Unspecific peroxygenases (UPOs) are a class of heme‐thiolate oxygenases from fungi that have similar catalytic scope to P450s, but are dependent only upon hydrogen peroxide (H2O2) as the external oxidant. A recent survey by Faiza and co‐workers explored the diversity of UPOs within sequence databases and was able to identify two major groups of enzymes: ‘long’ UPOs (Group I), typified by AaeUPO, of approximately 45 kDa molecular weight, and ‘short’ UPOs (Group II), typified by the enzyme from Marasmius rotula (MroUPO), which are of approximately 29 kDa. In this study, we have cloned the gene encoding an ‘artificial’ short UPO (artUPO) close in sequence to MroUPO, and expressed it in both Pichia pastoris and E. coli. In addition to their overall similarities in fold, artUPO, MroUPO and HspUPO feature both a glutamic acid and histidine residue (E164 and H93 in artUPO) that forms the catalytic acid‐base pair, in common with CPO and in contrast to the Glu‐Arg dyad found in AaeUPO.

We first crystallized artUPOyeast and determined the structure of the enzyme in two forms: the first in space group P212121, to a resolution of 2.01 Å and the second in C2221, to 1.21 Å, with two and one molecules in the asymmetric unit, respectively. The higher resolution structure in the C2221 space group superimposed with the monomer of the P212121 structure with an rmsd of 0.23 Å over 231 C‐alpha atoms, again indicative of high structural similarity, although clearly the higher resolution presents the enzyme structure in more detail with respect to water structure and alternate conformations of amino acids, which include D61 in the 1.21 Å structure. The structures confirm that each is a member of the short class of UPOs as defined by Faiza and co‐workers. The side chain amine of K156 H‐bonds with the backbone carbonyl groups of G89 and T90 in artUPOyeast, and may also confer extra stability to the enzyme. The differences between the active site tunnels of artUPOyeast and AaeUPO‐PaDa‐I are also noteworthy. artUPOyeast is distinguished from AaeUPO by the replacement of characteristic phenylalanine residues in that enzyme with smaller or hydrophilic side chains including I91 for F121, L65 for F76 and K156 for F188, with G195 (common to AaeUPO and HspUPO) replaced by L163. Catalytic efficiency for the UPO substrate 5‐nitro‐1,3‐benzodioxole (NBD) was largely the same for both enzymes, and the structures also revealed few differences apart from the expected glycosylation of the yeast enzyme.

> SQDIVDFSQHPWKAPGPNDLRSPCPGLNTLANHGFLPRNGRNITIPMIVQAGFDGYNVQPDILILAAKVGLLTSPEPDTFTLDDLKLHGTIEHDASLSREDFALGDNLHFNEAIFNTLANSNPGSDVYNITSAGQVLKDRLADSLARNPNVTNTGKEFTIRTLESAFYLSVMGNATTGEAPKNFVQIFFREERLPIEEGWKRSTTPITSDTLNPIAGQISEASNWKPNPDQCPWIVLSPNL> MLKHVAAALLLATAMPVVAQSPAPAAAPAPAARSIAATPPKLIVAISVDQFSADLFSEYRQYYTGGLKRLTSEGAVFPRGYQSHAATETCPGHSTILTGSRPSRTGIIANNWFDLDAKREDKNLYCAEDESQPGSSSDKYEASPLHLKVPTLGGRMKAANPATRVVSVAGKDRAAIMMGGATADQVWWLGGPQGYVSYKGVAPTPLVTQVNQAFAQRLAQPNPGFELPAQCVSKDFPVQAGNRTVGTGRFARDAGDYKGFRISPEQDAMTLAFAAAAIENMQLGKQAQTDIISIGLSATDYVGHTFGTEGTESCIQVDRLDTELGAFFDKLDKDGIDYVVVLTADHGGHDLPERHRMNAMPMEQRVDMALTPKALNATIAEKAGLPG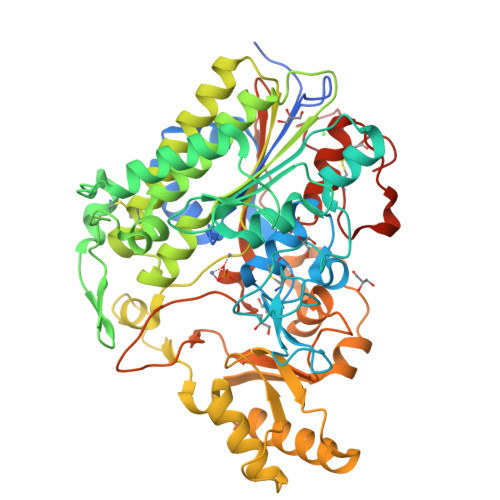KKVIWSDGPSGDIYYDKGLTAAQRARVETEALKYLRAHPQVQTVFTKAEIAATPSPSGPPESWSLIQEARASFYPSRSGDLLLLLKPRVMSIPEQAVMGSVATHGSPWDTDRRVPILFWRKGMQHFEQPLGVETVDILPSLAALIKLPVPKDQIDGRCLDLVAGKDDSCAGQLEHHHHHH>[2x]MEVEKEFITDEAKELLSKDKLIQQAYNEVKTSICSPIWPATSKTFTINNTEKNCNGVVPIKELCYTLLEDTYNWYREKPLDILKLEKKKGGPIDVYKEFIENSELKRVGMEFETGNIS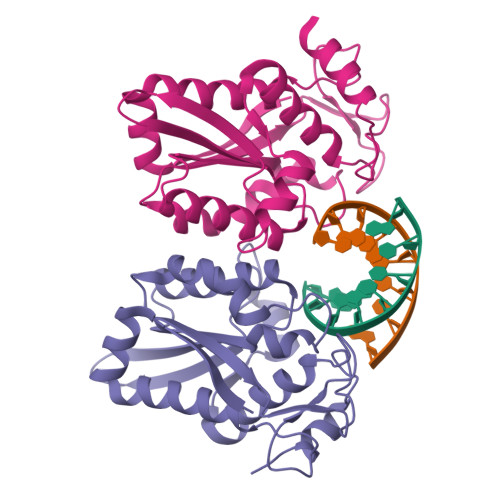SAHRSMNKLLLGLKHGEIDLAIILMPIKQLAYYLTDRVTNFEELEPYFELTEGQPFIFIGFNAEAYNSNVPLIPKGSDGMSKRSIKKWKDKVENK> GMSSIGLAHNVTILGSGETTVVLGHGYGTDQSVWKLLVPYLVDDYKVLLYDHMGAGTTNPDYFDFDRYSSLEGYSYDLIAILEEFQVSKCIYVGHSMSSMAAAVASIFRPDLFHKLVMISPTPRLINTEEYYGGFEQK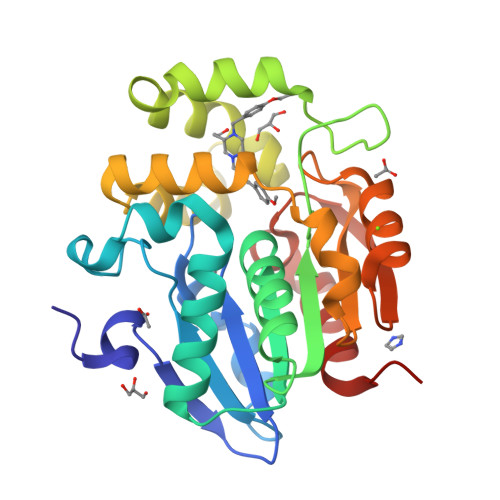VMDETLRSLDENFKSLSLGTAPLLLACDLESAAMQEYCRTLFNMRPDIACCITRMICGLDLRPYLGHVTVPCHIIQSSNDIMVPVAVGEYLRKNLGGPSVVEVMPTEGHLPHLSMPEVTIPVVLRHIRQDITDH>[2x]VPFCGHIKGGMRPGKKVLVMGIVDLNPESFAISLTCGDSEDPPADVAIELKAVFTDRQLLRNSCISGERGEEQSAIPYFPFIPDQPFRVEILCEHPRFRVFVDGHQLFDFYHRIQT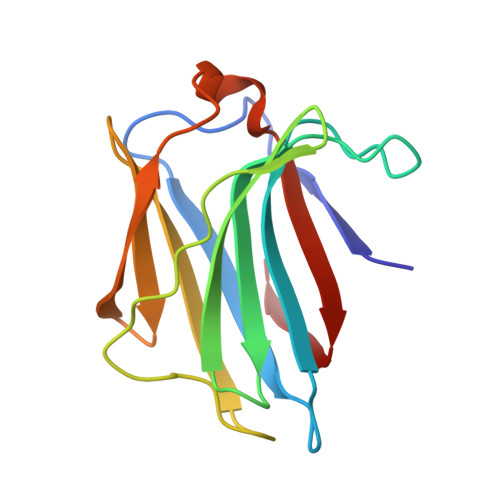LSAIDTIKINGDLQITKL[(2R,3S,4R,5R)-5-(2,4-dioxo-3,4-dihydropyrimidin-1(2H)-yl)-3,4-dihydroxytetrahydrofuran-2-yl]methyl (2S,3R,4S,5S)-3,4,5-trihydroxytetrahydro-2H-pyran-2-yl 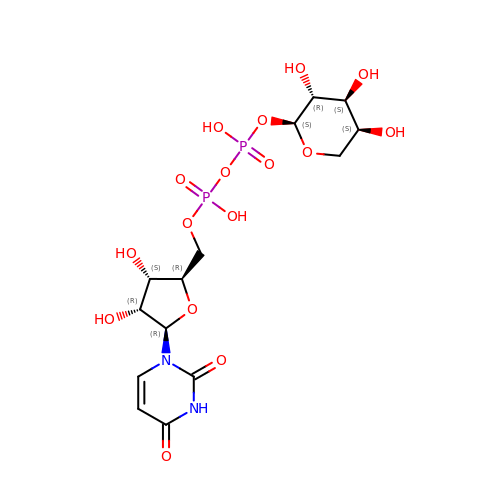dihydrogen diphosphate | C14 H22 N2 O16 P2 | DQQDLYVHOTZLOR-YDXBSWQDSA-N> QAEEWYFGKITRRESERLLLNPENPRGTFLVRESETTKGAYCLSVSDFDNAKGLNVKHYKIRKLDSGGFYITSRTQFSSLQQLVAYYSKHADGLCHRLTN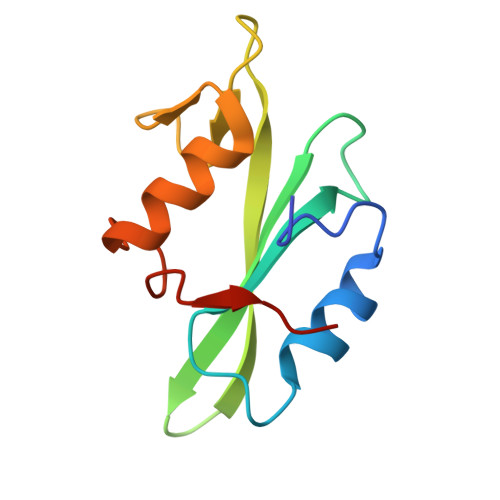VCPTSK>[2x]GHMTEIE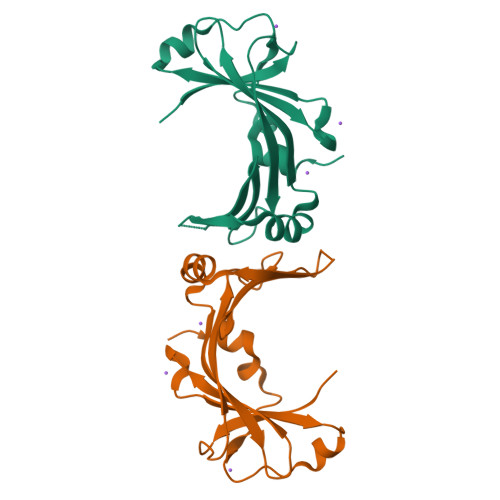RKFLVATFPDGELHAVPLRQGYLTTPTDSIELRLRQQGTEYFMTLKSEGGLSRQEYEIQIDVTQFEMLWPATEGRRVEKTRYSGKLPDGQLFELDVFAGHLSPLMLVEVEFLSEDAAQAFIPPPWFGEEVTEDKRYKNKALALSIP>[4x]GPLGSPEFSPLLQPGLAELRRRVQEAGVPQTPQPLTDAFLLRFLRARDFDLDLAWRLMKNYYKWRAECPELSADLRPRSILGLLKAGYHGVLRSRDSTGSRVLIYRIAYWDPKVFTAYDVFRVSLITSELIVQEVETQRNGVKAIFDLEGWQVSHAFQITPSVAKKIAAVLTDSFPLKVRGIHLINEPVIFHAVFSMIKPFLTEKIKDRIHLHGNNYKSSMLQHFPDILPREYGGKEFSMED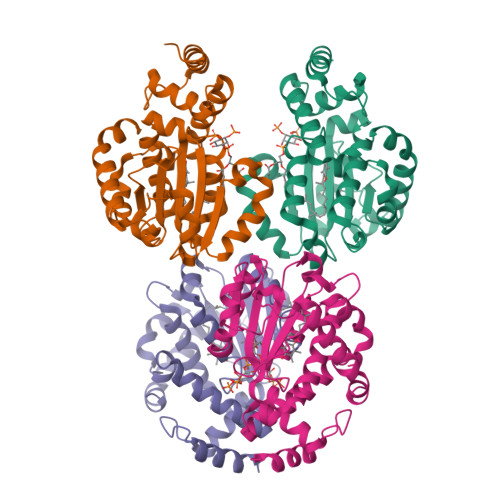ICQEWTNFIMKSEDYLSSISETIQ> MKTEWPELVGKSVEEAKKVILQDKPAAQIIVLPVGT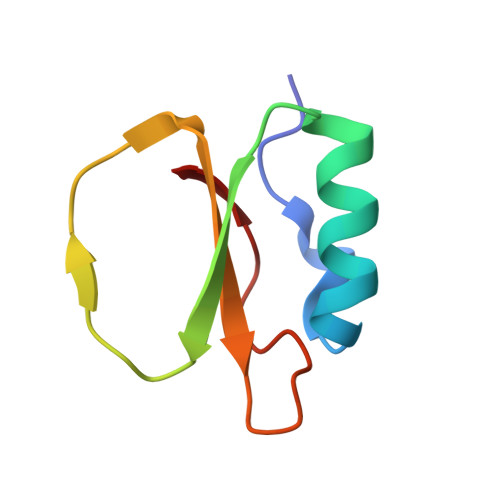IVPMEYRIDRVRLFVDRLDNIAQVPRVG>MRDPFMEALGLKVLHLAPGEAVVAGEV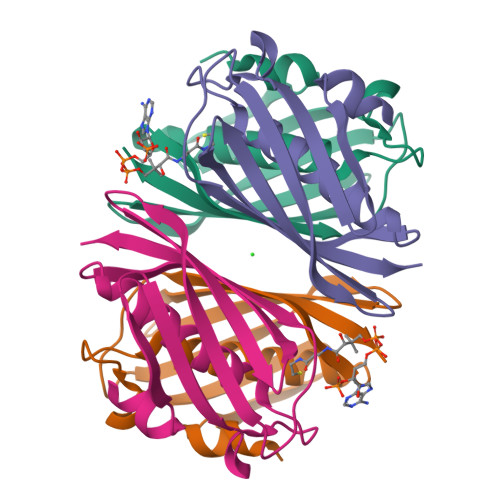RADHLNLHGTAHGGFLYALADSAFALASNTRGPAVALSCRMDYFRPLGAGARVEARAVEVNLSRRTATYRVEVVSEGKLVALFTGTVFRLGGDGDDVPAGTGNLAPREA[8x]>[2x]MSSVSLQDFDAERIGLFHEDIKRKFDELKSKNLKLDLTRGKPSSEQLDFADELLA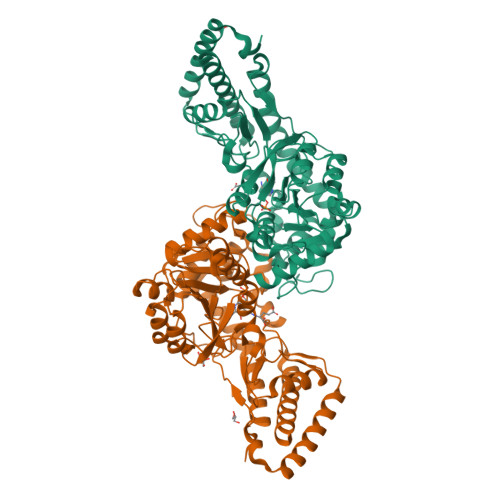LPGKGDFKAADGTDVRNYGGLDGIVDIRQIWADLLGVPVEQVLAGDASSLNIMFDVISWSYIFGNNDSVQPWSKEETVKWICPVPGYDRHFSITERFGFEMISVPMNEDGPDMDAVEELVKNPQVKGMWVVPVFSNPTGFTVTEDVAKRLSAMETAAPDFRVVWDNAYAVHTLTDEFPEVIDIVGLGEAAGNPNRFWAFTSTSKITLAGAGVSFFLTSAENRKWYTGHAGIRGIGPNKVNQLAHARYFGDAEGVRAVMRKHAASLAPKFNKVLEILDSRLAEYGVAQWTVPAGGYFISLDVVPGTASRVAELAKEAGIALTGAGSSYPLRQDPENKNLRLAPSLPPVEELEVAMDGVATCVLLAAAEHYANHHHHHH> MIIYGVYIVSKSGGLIFNLDNNVPRIEHEKTFTYPLDLVLDYDSKKVS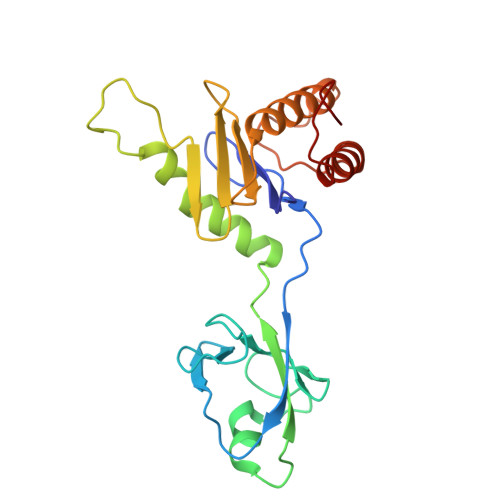VSFNRKDGINVGHVLVAVNGMPVNGVTLDDGRDVRTTLDAPENYPINLKFSRPKMTTNEKIFLASMFYPLFAIASQLSPEPKSSGIEILEADTFTLHCFQTLTGIKFIIISETGLNGIDLLLRKVYELYSDYVLKNPFYSLEMPIRCELFDNKLQELLAQVEKTGISNIDK> MSMLKREDWYDLTRTTNWTPKYVTENELFPEEMSGARGISMEAWEKYDEPYKITYPEYVSIQREKDSGAYSIKAALERDGFVDRADPGWVSTMQLHFGAAALEEYAASTAEARMARFAKAPGNRNMATFGMMDENRHGQIQLYFPYANVKRSRKWDWAHKAIHTNEWAAIAARSFFDDMMMTRDSVAVSIMLTFAFETGFSNMQFLGLAADAAEAGDHTFASLISSIQTDESRHAQQGGPSLKILVENGKKDEAQQMVDVAIWRSWKLFSVLTGPIMDYYTPLESRNQSFKEFMLEWIVAQFERQLLDLGLDKPWYWDQFMQDLDETHHGMHLGVWYWRPTVWWDPAAGVSPEEREWLEEKYPGWNDTWGQCWDVITDNLVNGKPELTVPETLPTICNMCNLPIAHTPGNKWNVKDYQLEYEGRLYHFGSEADRWCFQIDPERYKNHTNLVDRFLKGEIQPADLAGALMYMSLEPGVMGDDAHDYEWVKAYQKKTNAA;> MSEQQPEALKPLKTWSHLAGNRRRPSEYEVVSTNLHYFTDNPERPWELDSNLPMQTWYKKYCFDSPLKHDDWNAFRDPDQLVYRTYNLLQDGQESYVQGLFDQLNDRGHDQMLTREWVETLARFYTPARYLFHALQMGSVYIHQIAPASTITNCATYETADHLRWLTHTAYRTRELANCYPDVGFGKRERDVWENDPAWQGFRELIEKALIAWDWGEAFTAIN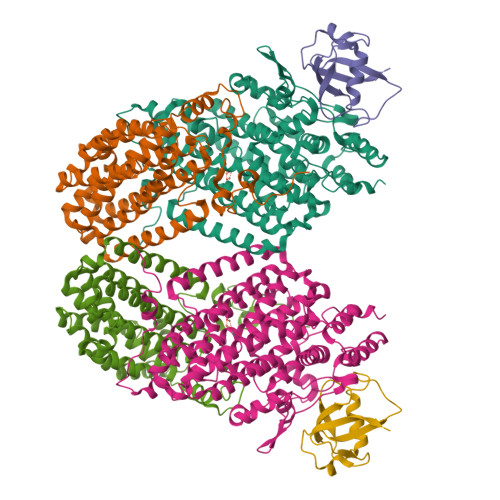LVTKPAVEEALLQQLGSLAQSEGDTLLGLLAQAQKRDAERHRRWSSALVKMALEKEGNREVLQKWVAKWEPLADKAIEAYCSALPDGENAIVEAKSASRYVRQMMGL;> MATFPIMSNFERDFVIQLVPVDTEDTMDQVAEKCAYHSINRRVHPQPEKILRVRRHEDGTLFPRGMIVSDAGLRPTETLDIIFMDN methyl radical | C H3 | 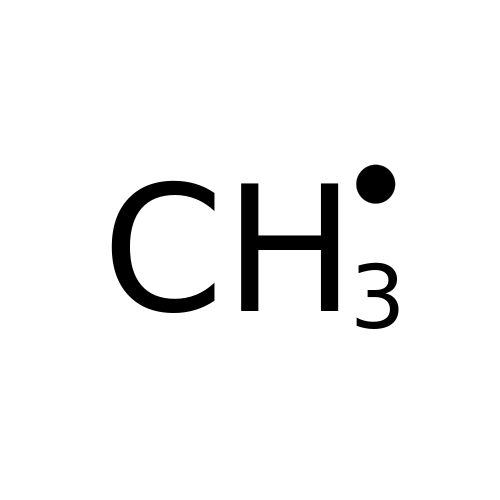VNWKTOKETHGBQD-UHFFFAOYSA-N> GAMSRQANRGTESKKMSSELFTLTYGALVTQLCKDYENDEDVNKQLDRMGYNIGVRLIEDFLARSNVGRCHDFRETADVIAKVAFKMYLGITPSITNWSPAGDEFSLILENNPLVDFVELPDNHSALIYSNLLCGVLRGALEMVQMAVEAKFVQDTLKGDGVTEIRMRFIRRIEDNLPA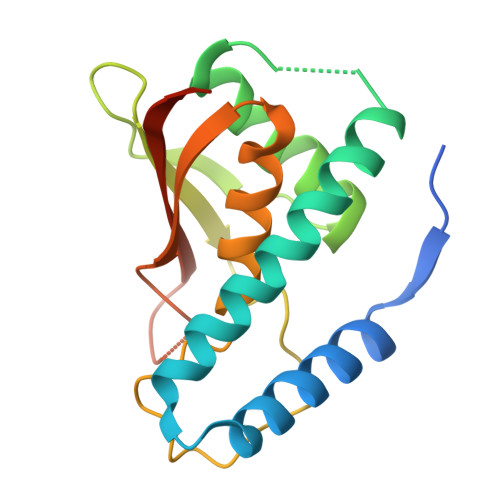GEE>EVDPRLYFENRSKFIQDQKDKGINPYPHKFERTISIPEFIEKYKDLGNGEHLEDTILNITGRIMRVSASGQKLRFFDLVGDGEKIQVLANYSFHNHEKGNFAECYDKIRRGDIVGIVGFPGKSKKGELSIFPKETILLSACLHMLPMKYGLKDTEIRYRQRYLDLLINESSRHTFVTRTKIINFLRNFLNERGFFEVETPMMNLIAGGANARPFITHHNDLDLDLYLRIATELPLKMLIVGGIDKVYEIGKVFRNEGIDNTHNPEFTSCEFYWAYADYNDLIKWSEDFFSQLVYHLFGTYKISYNKDGPENQPIEIDFTPPYPKVSIVEEIEKVTNTILEQPFDSNETIEKMINIIKEHKIELPNPPTAAKLLDQLASHFIENKYNDKPFFIVEHPQIMSPLAKYHRTKPGLTERLEMFICGKEVLNAYTELNDPFKQKE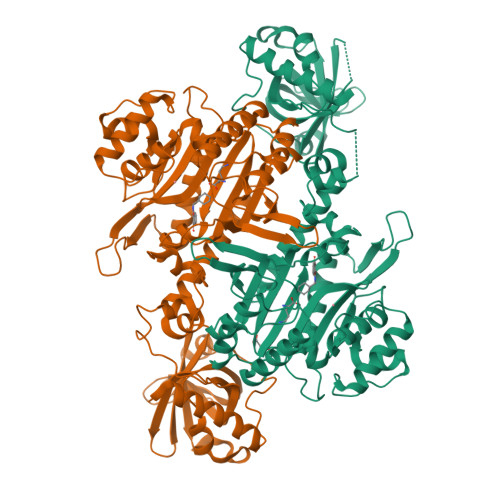CFKLQQKDREKGDTEAAQLDSAFCTSLEYGLPPTGGLGLGIDRITMFLTNKNSIKDVILFPTMRPAN[4x]> MNTVRSEKDSMGAIDVPADKLWGAQTQRSLEHFRISTEKMPTSLIHALALTKRAAAKVNEDLGLLSEEKASAIRQAADEVLAGQHDDEFPLAIWQTGSGTQSNMNMNEVLANRASELLGGVRGMERKVHPNDDVNKSQSSNDVFPTAMHVAALLALRKQLIPQLKTLTQTLNEKSRAFADIVKIGRTHLQDATPLTLGQEISGWVAMLEHNLKHIEYSLPHVAELALGGTAVGTGLNTHPEYARRVADELAVITCAPFVTAPNK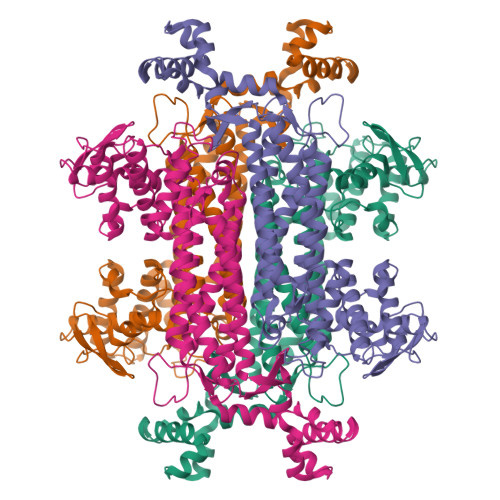FEALATCDALVQAHGALKGLAASLMKIANDVRWLASGPRCGIGEISIPENEPGSSIMPGKVNPTQCEALTMLCCQVMGNDVAINMGGASGNFELNVFRPMVIHNFLQSVRLLADGMESFNKHCAVGIEPNRERINQLLNESLMLVTALNTHIGYDKAAEIAKKAHKEGLTLKAAALALGYLSEAEFDSWVRPEQMVGSMKAGR> MTRLRSLYACMTNGWPVLLALILQAPAAQAEPGAEPIHRVSSELCANCHEDIYRQWKGSMHAKSTALSDPIHGLFYQQEVGDPTAEGMVHKKSGKFPLCLYCHAPNAARDQTTKLDAHPAYTEGVNCVACHTLKTYNGIQDAEGKLRYGIKAYDLSDRLQAPIGFPRELERLKARSDDLFGGAVDAVPDQKPNPHLGEPVELDGKTIPALTMEANPRQLRTSDACMGCHDQRDNPQGVPLCQTGKEFIAGGSQVACQTCHMPVAGGFADHSMGGGHHEAMLKRSIVFDLTTKADKEKIAAQVWIRNLQPHAMPTGAPFRNLYLKLTAYDASGEVLWQNAADHPSKDDPRAYFAYGLADDQGNPAPPPTATKPGDDTRLQPHETRELN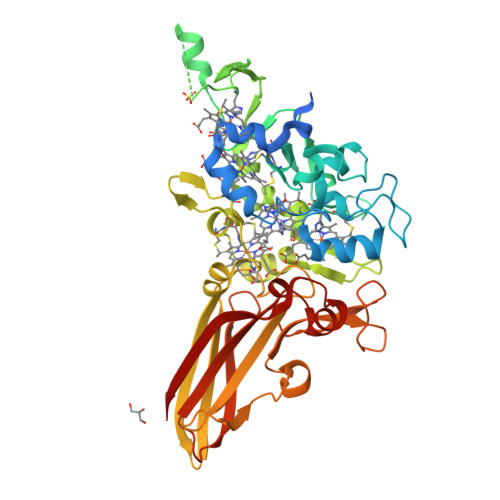YEIPAKGVALVRGELYYNLLWPSLVEKFTQLPAELTAPVLIAVSEKPI> MSEQKQDVAATEEQQPVLQIQRIYVKDVSFEAPNLPHIFQQEWKPKLGFDLSTETTQVGDDLYEVVLNISVETTLEDSGDVAFICEVKQAGVFTISGLEDVQMAHCLTSQCPNMLFPYARELVSNLVNRGTFP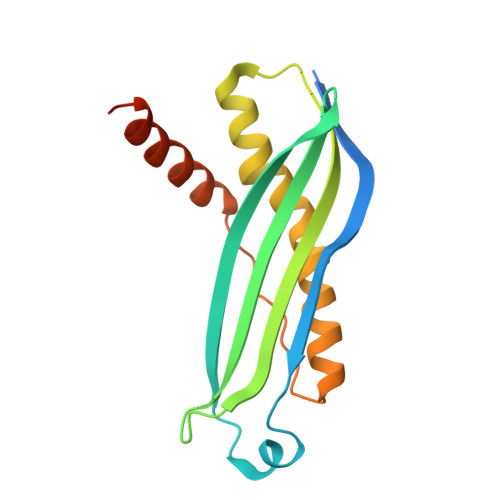ALNLSPVNFDALFVEYMNRQQAENAEEKSEEEQTKH ethyl (5S,8S,14S)-14-hydroxy-5,8,11-tris(2-methylpropyl)-3,6,9,12-tetraoxo-1-phenyl-2-oxa-4,7,10,11-tetraazapentadecan-15-oate 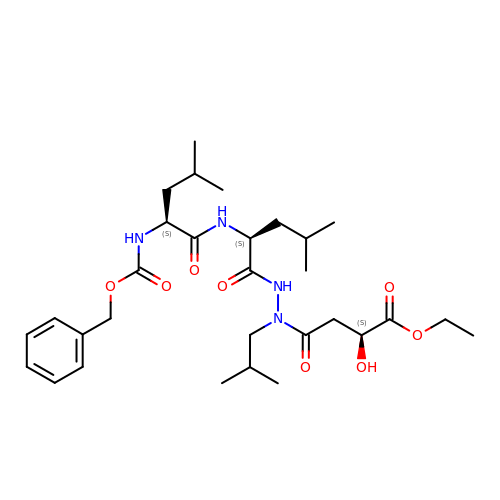| C30 H48 N4 O8 | DDKYUZVIGXLULX-SDHOMARFSA-N>[2x]MRDHRKIGKQLDLYHMQEEAPGMVFWHNDGWTIFRELEVFVRSKLKEYQYQEVKGPFMMDRVLWEKTGHWDNYKDAMFTTSSENREYCIKPMNCPGHVQIFNQGLKSYRDLPLRMAEFG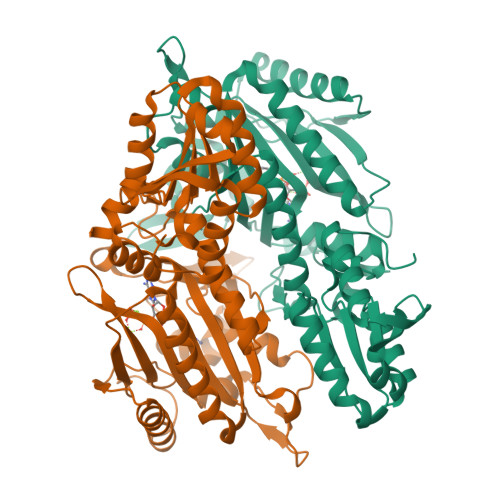SCHRNEPSGSLHGLMRVRGFTQDDAHIFCTEEQIRDEVNGCIRLVYDMYSTFGFEKIVVKLSTRPEKRIGSDEMWDRAEADLAVALEENNIPFEYQLGEGAFFGPKIEFTLYDCLDRAWQCGTVQLDFSLPSRLSASYVGEDNERKVPVMIHRAILGSMERFIGILTEEFAGFFPTWLAPVQVVIMNITDSQSEYVNELTQKLSNAGIRVKADLRNEKIGFKIREHTLRRVPYMLVCGDKEVESGKVAVRTRRGKDLGSMDVNEVIEKLQQEIRSRSLKQLEELEHHHHHH>GPLGSPEFGRPGWVIGVDPDIGGAIAVLSPDGSSQVFDNPFVHIVVSEVIRKRLDTKSIIQLLRGLDAPPGTTAYIEKSSPFPTDGKQGWWSTGFSYGLWIASLVASGFSVVPIASQTWKAYFGLMRSETPKDDSRQAASILFPDKDQSLK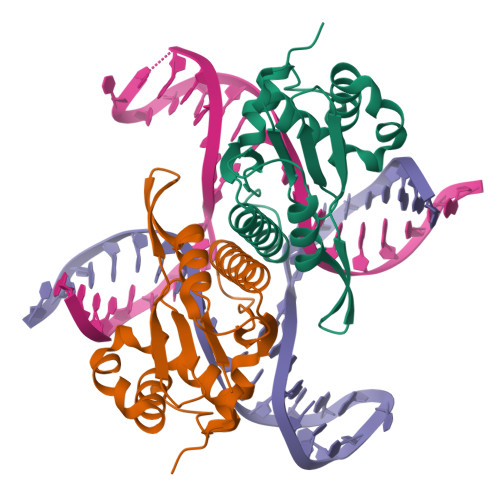LKKHAGRAEALLLAAYGKGLVLP[2x]> MAAPQFHRPSTITADNVRALGTRGLVLATNNAQFIMDNS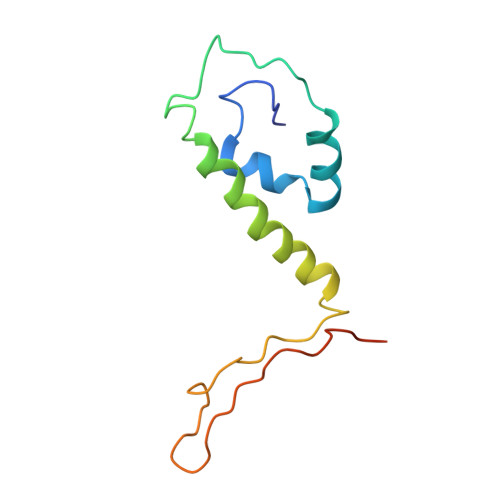YPHPHGTQGAVREFLRGQAAALTDLGVTHANNTFAPQPMFAGDAAAEWLRPSFGLKRTYSPFVVRDPKTPSTP>[8x]MDYKDDDDKNRALSPMVSEFETIEQENSYNEWLRAKVATSLADPRPAIPHDEVERRMAERFAKMRKERSKQ;>[8x]MLPVLWLESA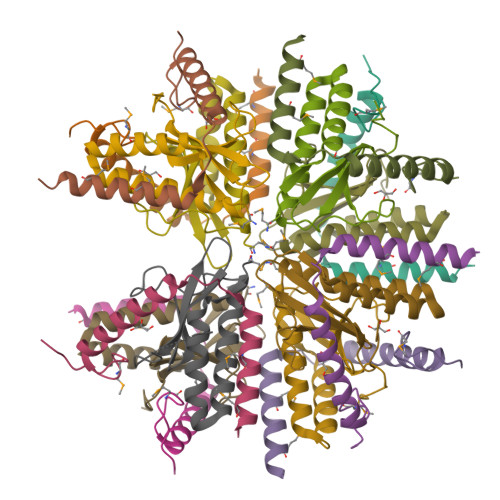DTDLDDITSYIARFDIDAAERLWQRLRGCVLPLSEHPYLYPPSDRVPGLREIVAHPNYIILYRVTTSSVEVVNVIHARRQFPLEHHHHHH>[4x]GSHMASMTGGQQMGRGSGQQMETGDQRFGDLVFRQLAPNVWQHTSYLDMPGFGAVASNGLIVRDGGRVLVVDTAWTDDQTAQILNWIKQEINLPVALAVVTQAHQDKMGGMDALHAAGIATYANALSNQLAPQEGMVAAQHSLTFAANGWVEPATAPNFGPLKVFYPGPGHTSDNITVGIDGTDIAFGGCLIKDSKAKSLGNLGDADTEHYAASARAFGAAFPKASMIVM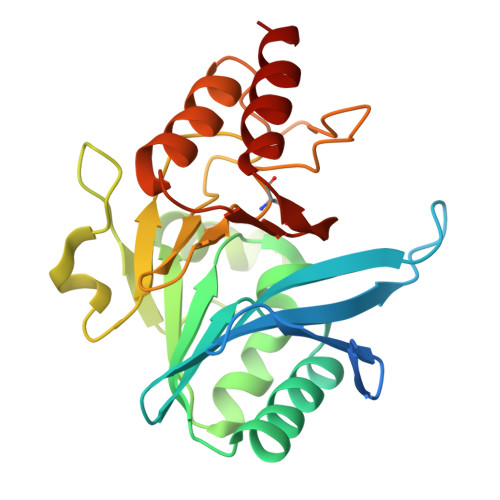SHSAPDSRAAITHTARMADKLR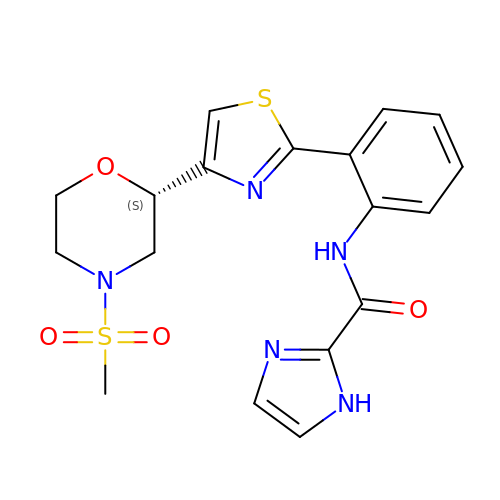N-(2-{4-[(2S)-4-(methylsulfonyl)morpholin-2-yl]-1,3-thiazol-2-yl}phenyl)-1H-imidazole-2-carboxamide | C18 H19 N5 O4 S2 | MPCBXJASUBLGMA-HNNXBMFYSA-N>MENSFKAALKAGRPQIGLWLGLSSSYSAELLAGAGFDWLLIAGEHAPNNVQTVLTQLQAIAPYPSQPVVRPSWNDPVQIKQLLDVGTQTLLVPMVQNADEAREAVRATRYPPAGIRGVGSALARASRWNRIPDYLQKANDQMCVLVQIETREAMKNLPQILDVEGVDGVFIGPADLSADMG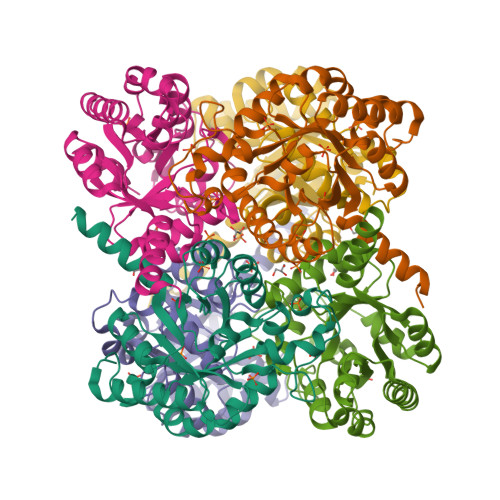YAGNPQHPEVQAAIEQAIVQIRESGKAPGILIANEQLAKRYLELGALFVAVGVDTTLLARAAEALAARFGAQATAVKPGVY[2x]>[4x]GSSHHHHHHSGDPASMNNHPEVKIKTILSLFLNINIDDFNMDANLADAYDMDSTELADLAKEIEKEFGISVTKSQFSHWETGRAVLDFVSSSLNDKN;>[4x]GSSHHHHHHSGDPASMIINNRNESQPRRVVVTGLGVVAPTGVGVNEFWNNIHNGKSG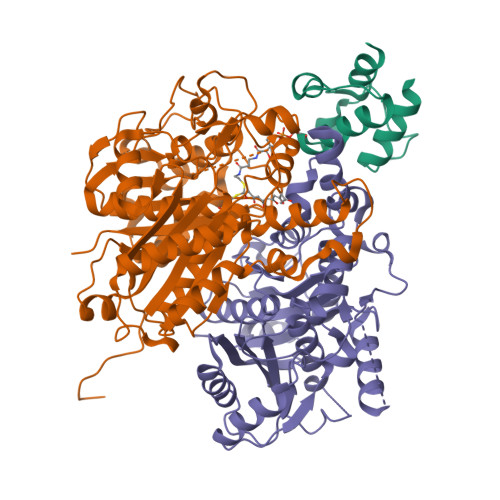VSKYEWGRERFGFKSGAIGQVYGSDGNNKEFVLKSERKYLQFALDAAEMAMQDANLRPSDIDGRRFGVAIATAIADAAGMEECLLRITKGGKENIHPDLIKSEDYDSFDFSSAATSVAKKYGASMSVSNISTGCAAGLDALGIAMEHIRYGRADIMLAGASEAPLCPLSIGSFEALGALSSRELENQQAATCPFSLERDGFVIAEGCGILILESYEHAKQRGAHIYAELAGYASVNNAYHMTDLPADGMAMARCIDMALKDAQISPSTVNYISAHGSSTAQNDINESNAIKFVLGESAFGIPINSLKSMTGHALAAANAIESVALCLEIEKQYVHPTINYQTPDPDCDLDYIPNQGCSYPIKTALKLSSGFSGIHSVIVMRAVDNA;>MRKRVVVTGVGAIHPDGNDVTAIKSKVIQKLLGQESKNNTTASSIIRTLSDFDGAKYINNRLRRKIDEFSVYGIVAVEMALKASRLDVDKLDPNRVGIYVGNCFGGWQHIEDEVKALHIEGIKGMGPYVATAWFPAALQGQLSLLYGFSAQSKTFSTSDVAGMQAIGYAAEAISNGVAEVMLCGASEHLSSPLVKNLLEKTSSQKHSEVFGEKQPGDFSEGAAFLVLEERQHALERGASILCELTGFVDYFAPDKNTRNNTLEYTAELFNHNENAVFIMDGIYDDEKEITSKAFSNKEIKTSFINLRPYLDNQFSVSGVIDSVLASSFLSESHGDEEQQSKKINEFSNTNQIIIQRFSNQGHVCALSFSAI[4x]With No Lysine (WNK) kinases are soluble intracelluar serine–threonine kinases noted for their unique active site and their association with familial hyperkalemic hypertension (FHHt). WNKs are the chloride-inhibited protein kinases long anticipated to control the activity of cation chloride cotransporters in response to osmotic stress. WNKs are activated by osmotic stress in cells and are inhibited by chloride. A model for WNK regulation, then, is the presence of a dimer–monomer equilibrium: the dimer is inactive and binds inhibitory ligands; the monomer is autophosphorylation-competent.

WNK1/E388 (WNK3/E314) is noteworthy because it is on the Activation Loop that undergoes large conformational changes upon phosphorylation. Mutation of E314 in the Activation Loop of WNK3 (WNK3/E314Q and WNK3/E314A, and the homologous WNK1/E388A) enhanced the rate of autophosphorylation, and reduced chloride sensitivity. The high activity of the mutants WNK3/E314Q, WNK3/E314A, and WNK1/E388A suggests a loss of the CWN1-stabilized inhibitory conformation. To address whether conformational changes induced by the mutations correlate with the effects of PEG400, WNK3/SA/E314A and the corresponding WNK1/SA/E388A were crystalized. WNK3/SA/E314A crystallized, affording limited diffraction to 3.4 Å. WNK3/SA/E314A crystals were in space group P1, and adopts a unique dimer in which the Activation Loops are swapped. The significance of this domain swapping is unclear. Excluding the Activation Loops, comparisons of uWNK3/SA/E314A, uWNK1/SA, and uWNK1/SA/PEG400 show that uWNK3/SA/E314A is more similar to uWNK1/SA/PEG400 than uWNK1/SA (with r.m.s.d.’s of 0.7 versus 0.85, respectively). Furthermore, the orientations of the 3/10 helix and helix C most resemble WNK1/SA/PEG400. Crystallography of WNK3/E314A shows that it exhibits conformational differences at the same loci as observed by PEG400 applied to crystals of WNK1.

>EEEAEMKAVATSPSGRFLKFDIELGRGAFKTVYKGLDTETWVEVAWCELQDRKLTKAEQQRFKEEAEMLKGLQHPNIVRFYDSWESILKGKKCIVLVTELMTSGTLKTYLKRFKVMKPKVLRSWCRQILKGLQFLHTRTPPIIHRDLKCNNIFITGPTGSVKIGDLGLATLMRTSFAKSVIGTPAFMAPEMYEEHFDESVDVYAFGMCMLEMATSEYPYSECQNAAQIYRKVTSGIKPASFNKVTDPEVKEIIEGCIRQNKSERLSIRDLLNHAFFAEDT[2x]In this study, we apply a novel rational design approach to the stabilization of wild-type Amadoriase I from Aspergillus fumigatus. Using a rational in silico computational design and screening method, we have produced two forms of the deglycating enzyme Amadoriase I featuring a significantly higher thermostability compared to the WT enzyme. In particular, the introduction of disulfide bonds provide considerable stability to proteins by locking their fold in a well-defined local or global conformation. We used X-ray crystallography to confirm the introduction of the designed disulfide bonds in the mutant enzymes.

To confirm the formation of the designed disulfide bond in the SS03 and in the SS17 mutants and to assess any possible change that such modifications may have caused to their global molecular architecture relative to the wild-type enzyme, we solved the crystal structures of these two thermostabilized species. The crystal structures of the SS03 and the SS17 mutants were determined at 2.15 and 2.85 Å resolution, respectively. Focusing on the region where the mutations were introduced, the SS03 mutant (S67C/P121C) is highly superimposable to the wild type enzyme (residues 62 to 72 and 116 to 126, RMSD = 0.842) while the SS17 variant (D295C/K303C) shows a structural rearrangement in the region from residue 290 to 308, with an RMSD of 1.657 Å. Interestingly, while the introduction of the disulfide bond in the SS03 mutant does not cause any significant structural rearrangement in any portion of the enzyme, the formation of the disulfide bond in the SS17 mutant affects the conformation of one of the loops that define the boundaries of the tunnel leading to the catalytic pocket (residues 63 to 69) (orange circle). The RMSD between the SS17 mutant and the wild type enzyme for this short region is 2.745 Å. For the SS03 and the SS17 species, the mutations did not significantly affect the apparent steady state parameters relative to the WT. The SS17 variant, which shows an increase of ~8 °C in the T50 value and, contrary to all other tested mutants, a gradual decrease in residual activity at increasing temperatures, features detectable activity even after thermal treatment at 95 °C.

>[2x]HHHHHHSSGHIDDDDKMAPSILSTESSIIVIGAGTWGCSTALHLARRGYKDVTVLDPHPVPSPIAAGNDINKIMEHSELKDGSSDPRSAAFSTFTRAALKAWKTDPVFQPYFHETGFIISGHTPALIDHIRKDEVEPSETNFVKLETAEDFRRTMPPGVLTGDFPGWKGWLHKSGAGWIHAKKAMISAFNEAKRLGVRFVTGSPEGNVVSLVYEDGDVVGARTADGRVHKAHRTILSAGAGSDSLLDFKKQLRPTAWTLCHIQMGPEEVKQYRNLPVLFNIAKGFFMEPDEDKHELKICDEHPGYCNFLPCPNRPGQECSVPFAKHQIPLEAEARARDFLHDTMPHLADRPLSFARICWDADTPDRAFLIDRHPEHPSLLVAVGGSGNGAMQMPTIGGFIADALESKLQKEVKDIVRWRPETAVDRDWRATQNRFGGPDRIMDFQQVGEDQWTKIGESRGP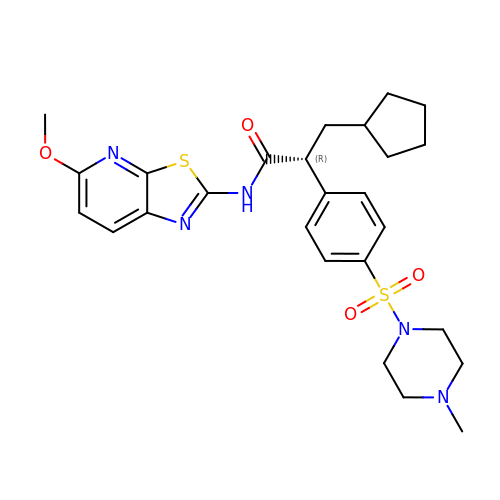(2R)-3-cyclopentyl-N-(5-methoxy[1,3]thiazolo[5,4-b]pyridin-2-yl)-2-{4-[(4-methylpiperazin-1-yl)sulfonyl]phenyl}propanamide | C26 H33 N5 O4 S2 | GMGMDWSPSKXMJH-OAQYLSRUSA-N> MEEFEKILEEIDSANLSQNAVQQLKQLIISNGILDDEQLMEKWLFQLEAIIYNSKQKFLEAQLMDFKKNVL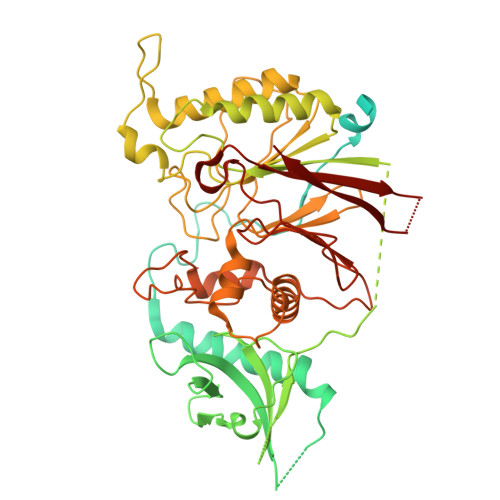NQDIKKPQNDNFKKIKESEVQKNIDIIKGDADLFTKASSAKKQTSTQQANNAAIDCEEQLRQQLGKESMLDPKRFSYNSNLPQVNFEKNQHQNSNNMTIVDLFEQYDPNKIPNYLTNNIDKIRKHLEQRILTFKIQNYSQFIVNGEQLINDVSSYSKTEEVKMVGRLISTENGFLNTTNLRIELNRNQYFDLVFENDFDFGNNVLFPNQIVMVKGIINEKEELVVSELITDHIKEITDEEHPKIDNLNQDESQLIMVAAGPFSTVMSTQYTSFDNILHVAKTKKVSTLILLGPFLDIKNEILKDGSIIINSKEYTFEQLQNSLFEKAVKELEGKTQIIIVPSTRDILSTDSIPQMSLEIKVSEHKNSIHSYSNPAYIDIDKLRVYIANSDVGMITLQNSLLDKKIPYMQQSRLTFKALMNQQNLYSIYPMRNPQDSQQILETVKLPNINDFDIPFDYQLEQYPHIIISPSSLPKFATKIYNTVVINPNYVIRDGSQAGNFAIITLFKDSDIPIHERTRVDLYCL> TIGMVVIHKTGHIAAGTSTNGIKFKIHGRVGDSPIPGAGAYADDTAGAAAATGNGDILMRFLPSYQAVEYMRRGEDPTIACQKVISRIQKHFPEF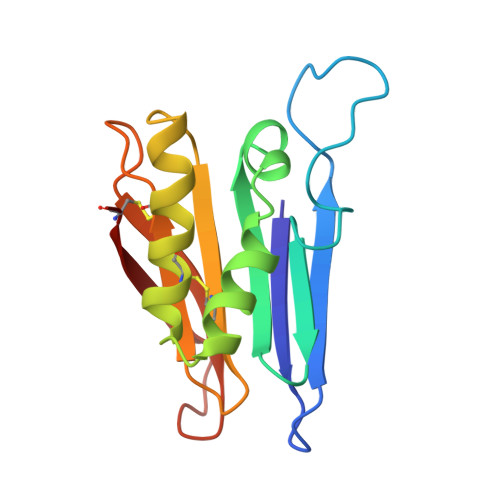FGAVICANVTGSYGAACNKLSTFTQFSFMVYNSEKNQPTEEKVDCI>[2x]HAHLKSATPAADSTVAAPADLRLTFSEGVEATFTKVSLSKDGTEVAIKGL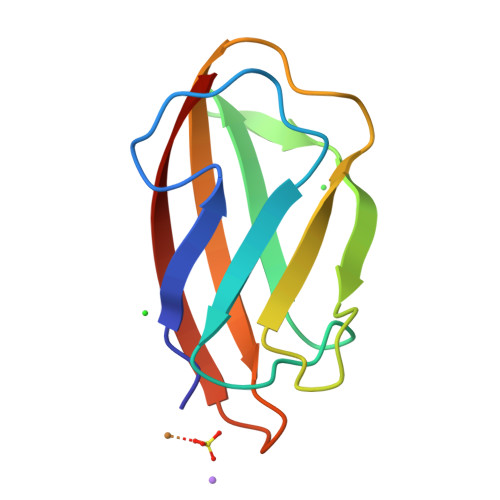ETPDADKKTLVVTPAAPLAAGNYKVVWNAVSVATHKSNGEYSFKVGQ>VHHHHHHPDYKDDDDKTYVQDKTPAFVCPAADIKTTKCLGPKDCLYPSPKTCNGYIQCSPADDSYLTGIIHEMPCPSGLLWNDNKKWCDWPENTTCGLVKSAGATEVDAT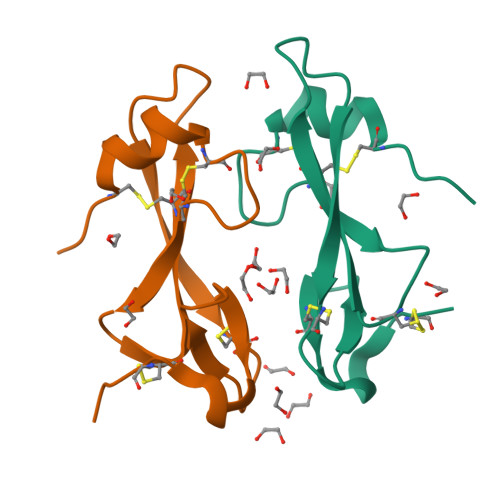KQGPTPGKYHG[2x]> MFKIVYPNAKDFFSFINSITNVTDSIILNFTEDGIFSRHLTEDKVLMAIMRIPKDVLSEYSIDSPTSVKLDVSSVKKILSKASSKKATIELTETDSGLKIIIRDEKSGAKSTIYIKAEKGQVEQLTEPKVNLAVNFTTDESVLNVIAADVTLVGEEMRISTEEDKIKIEAGEEGKRYVAFLMKDKPLKELSIDTSASSSYSAEMFKDAVKGLRGFSAPTMVSFGENLPMKIDVEAVSGGHMIFWIAPRL;> MKAKVIDAVSFSYILRTVGDFLSEANFIVTKEGIRVSGIDPSRVVFLDIFLPSSYFEGFEVSQEKEIIGFKLEDVNDILKRVLKDDTLILSSNESKLTLTFDGEFTRSFELPLIQVESTQPPSVNLEFPFKAQLLTITFADIIDELSDLGEVLNIHSKENKLYFEVIGDLSTAKVELSTDNGTLLEASGADVSSSYGMEYVANTTKMRRASDSMELYFGSQIPLKLRFKLPQEGYGDFYIAPRAD;> MIYLKSFERNIRLINMKVVYDDVRVLKDIIQALARLVDEAVLKFKQDSVELVALDRAHISLISVNLPREMFKEYDVNDEFKFGFNTQYLMKILKVAKRKEAIEIASESPDSVIINIIGSTNREFNVRNLEVSEQEIPEINLQFDISATISSDGFKSAISEVSTVTDNVVVEGHEDRILIKAEGESEVEVEFSKDTGGLQDLEFSKESKNS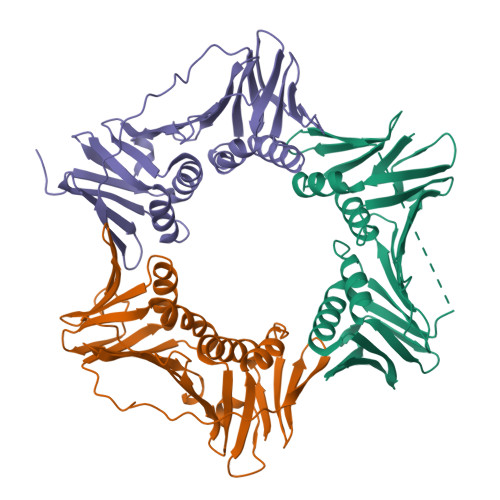YSAEYLDDVLSLTKLSDYVKISFGNQKPLQLFFNMEGGGKVTYLLAPKV>MGIMAASRPLSRFWEWGKNIVCVGRNYADHVREMRSAVLSEPVLFLKPSTAYAPEGSPILMPAYTRNLHHELELGVVMGKRCRAVPEAAAMDYVGGYALCL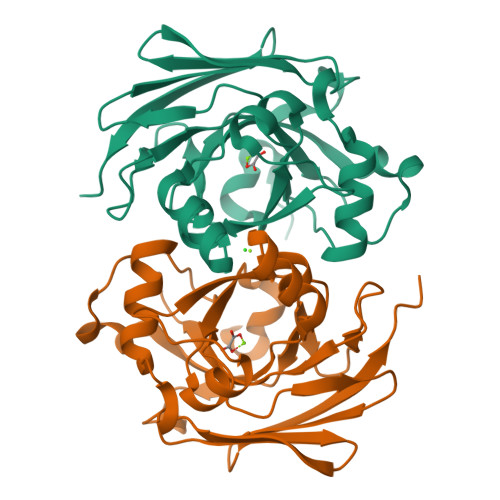DMTARDVQDECKKKGLPWTLAKSFTASCPVSAFVPKEKIPDPHKLKLWLKVNGELRQEGETSSMIFSIPYIISYVSKIITLEEGDIILTGTPKGVGPVKENDEIEAGIHGLVSMTFKVEKPEY[8x]> AQADIALIGLAVMGQNLILNMNDHGFVVCAFNRTVSKVDDFLANEAKGTKVLGAHSLEEMVSKLKKPRRIILLVKAGQAVDNFIEKLVPLLDIGDIIIDGGNSEYRDTMRRCRDLKDKGILFVGSGVSGGEDGARYGPSLMPGGNKEAWPHIKAIFQGIAAKVGTGEPCCDWVGDDGAGHFVKMVHNGIEYGDMQLICEAYHLMKDVLGLGHKEMAKAFEEWNKTELDSFLIEITASILKFQDADGKHLLPKIRDSAGQKGTGKWTAISALEYGVPVTLIGEAVFARCLSSLKDERIQASKKLKGPQNIPFEGDKKSFLEDIRKALYASKIISYAQGFMLLRQAATEFGWTLNYGGIALMWRGGCIIRSVFLGKIKDAFDRNPGLQNLLLDDFFKSA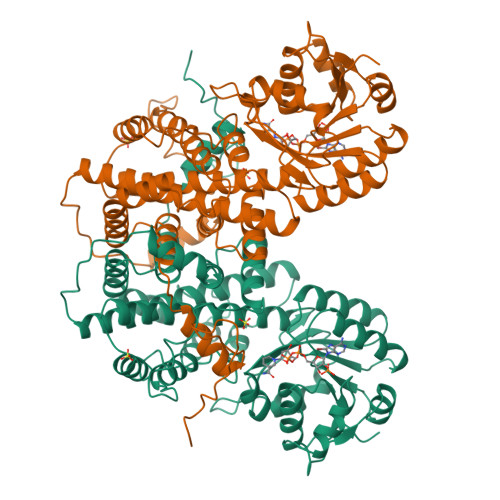VENCQDSWRRAISTGVQAGIPMPCFTTALSFYDGYRHAMLPANLIQAQRDYFGAHTYELLAKPGQFIHTNWTGHGGSVSSSSYNA> SSSPKITARWNPSEACRPLVDDAPIFYPTNEDFDDPLGYIEKLRSKAESYGICRIVPPVAWRPPCPLKEKKIWENSKFPTRIQFIDLLQNREPIKKSTKTKKRKRRRISKIGYTRRKRDSGCDTASSGSSDSEGKFGFQTGPDFTLAAFQKYDEYFKECYFQSEDHPGSKASENKKFKPKVKDLEGEYWRIVEQATDEVEVYYGADLETKKFGSGFPKYKPGYPISEADQYSQCGWNLNNLSRLPGSVLAFESCDISGVIVPWLYVGMCFSTFCWHVEDHHLYSMNYLHTGDPKVWYGIPGNHAESFENVM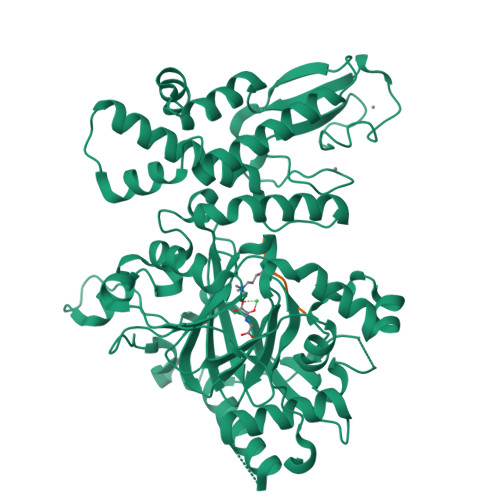KKRLPDLFEEQPDLLHQLVTQLSPRILKEEGVPVYRAVQRSGEFILTFPKAYHSGFNCGFNCAEAVNVAPVDWLVHGQNAVEGYSKQRRKSSLSHDKLLLGAAMEATYCLWELSLSKKKTPVIARWKRVCSEDGLLTKAVKKRVQMEEERLNHLQDGFSLRKMEGDFDNKRERECFLCFYDLHMSASSCKCSPNRFACLIHAKDLCSCESKDRYILIRHTLDELWALVRALEGDLDAIDLWASKCRDQYPSQH;> ARTKQTARKS> HMGSMEGKFYTSTEASEITHCSRRQLQYWREKGVIVPTVNSSGKGRNVYYSKADLLALTVMEQLLSTGLNFDLCYAALQTLRKQEPWLFDESVP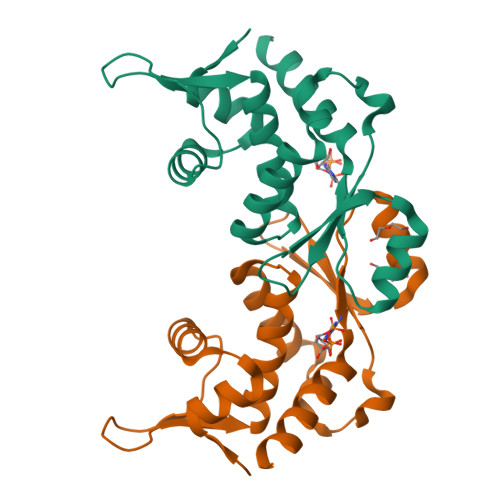EEKMKRLMLLPTRSPEQPLQLAEFDKQAALEALCHGQTVIPFWSDRIHQQLRENLKSFSS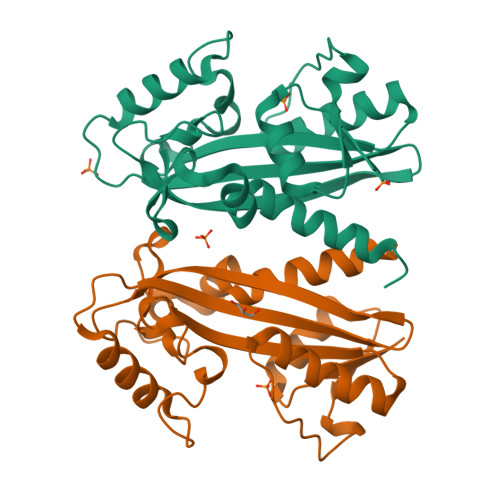>[2x]MKEIVIASNNQGKINDFKVIFPDYHVIGISELIPDFDVEETGSTFEENAILKSEAAAKALNKTVIADDSGLEVFALNGEPGIYSARYAGENKSDEANIEKLLNKLGNTTDRRAQFVCVISMSGPDMETKVFKGTVSGEIADGKYGENGFGYDPIFYVPKLDKTMAQLSKEQKGQISHRRNAINLLQAFLEGEKNV>[2x]MAVAELYTQYNRVWIPDPEEVWKSAEIAKDYRVGDKVLRLLLEDGTELDYSVNPESLPPLRNPDILVGENDLTALSYLHEPAVLHNLRIRFAESKLIYTYSGIILVAMNPYKQLPIYGDAII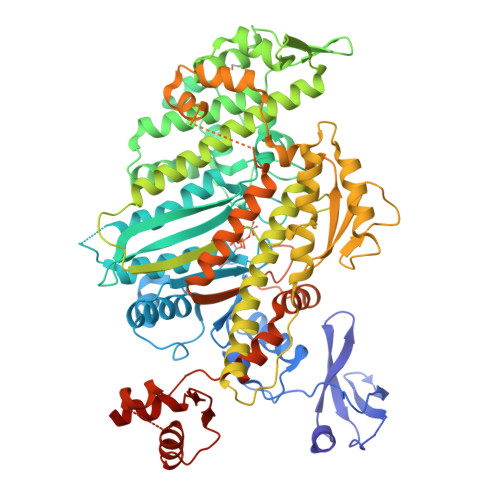HAYSGQNMGDMDPHIFAVAEEAYKQMARNNRNQSIIVSGESGAGKTVSARYAMRYFATVSKSGSNAHVEDKVLASNPITEAVGNAKTTRNDNSSRFGKYTEISFDEQNQIIGANMSTYLLEKSRVVFQSENERNYHIFYQLCASAQQSEFKHLKLGSAEEFNYTRMGGNTVIEGVNDRAEMVETQKTFTLLGFKEDFQMDVFKILAAILHLGNVQITAVGNERSSVSEDDSHLKVFCELLGLESGRVAQWLCNRKIVTSSETVVKPMTRPQAVNARDALAKKIYAHLFDFIVERINQALQFSGKQHTFIGVLDIYGFETFDVNSFEQFCINYANEKLQQQFNMHVFKLEQEEYMKEDIPWTLIDFYDNQPVIDLIEAKMGILELLDEECLLPHGTDENWLQKLYNNFVNRNPLFEKPRMSNTSFVIQHFADKVEYKCEGFLEKNRDTVYDMLVEILRASKFHLCANFFQENPTPPSPFGSMITVKSAKQVIKPNSKHFRTTVGSKFRSSLYLLMETLNATTPHYVRCIKPNDEKLPFEFDSKRIVQQLRACGVLETIRISAQSYPSRWTYIEFYSRYGILMTKQELSFSDKKEVCKVVLHRLIQDSNQYQFGKTKIFFRAGQVAYLEKLRLDKGDYKDDDDK>[16x]SAPGVPDARAIAAICEQLRQHVADLGVLYIKLHNYHWHIYGIEFKQVHELLEEYYVSVTEAFDTIAERLLQLGAQAPASMAEYLALSGIAEE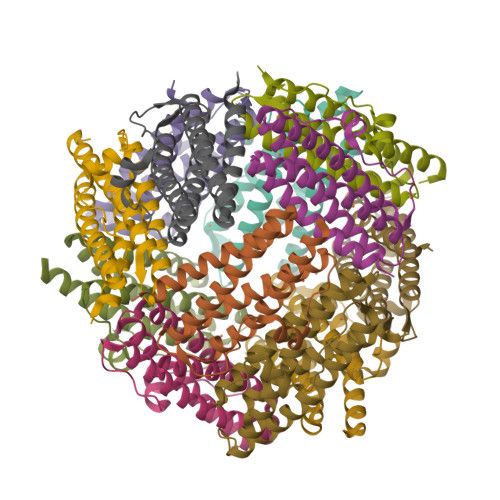TEKEITIVSALARVKRDFEYLSTRFSQTQVLAAESGDAVTDGIITDILRTLGKAIWMLGATLKA>MSDLKKAAQQAISLMDLTTLNDDDTDQKVIELCHKAKTPAGDTAAICIYPRFIPIARKTLNEIGGDDIKIATVTNFPHGNDDIAIAVLETRAAVAYGADEVDVVFPYRALMEGNETVGFELVKACKEACG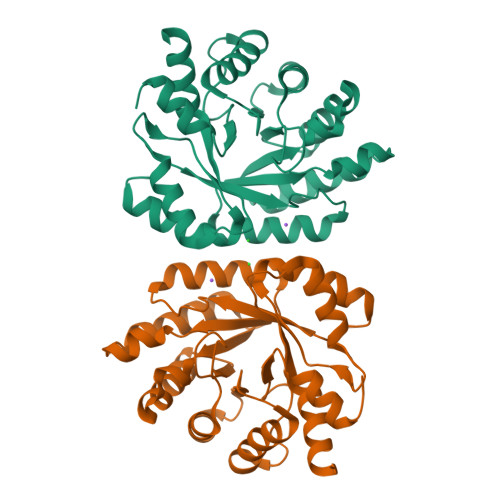EDTILKVIIESGVLADPALIRKASELSIDAGADFIKTSTGKVAVNATLEAAEIMMTVISEKNPKVGFKPAGGVKDAAAAAEFLGVAARLLGDDWATPATFRFGASSLLTNLLHTLELADAPQGAQGYLEHHHHHH[4x]N-[(E)-3-[(2R,3S,4R,5R)-3,4-dihydroxy-5-(6-propylaminopurin-9-yl)oxolan-2-yl]prop-2-enyl]-5-(4-fluorophenyl)-2,3-dihydroxy-benzamide 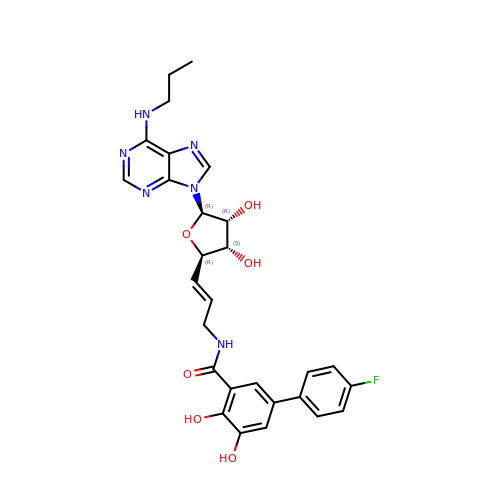| C28 H29 F N6 O6 | ZTSZMLSDNBUFMA-WIRSHZJASA-N>[9x]SELDSENDAADIAAGTIIAGAELTFGLLQNLLYFFANVNRKCAVGVDNESGFRWQEGSTYFFSGTADENLPYSVSDGYAVLYGPRKTNGPVATGVVGVLAYYIPSIGKTLAVMW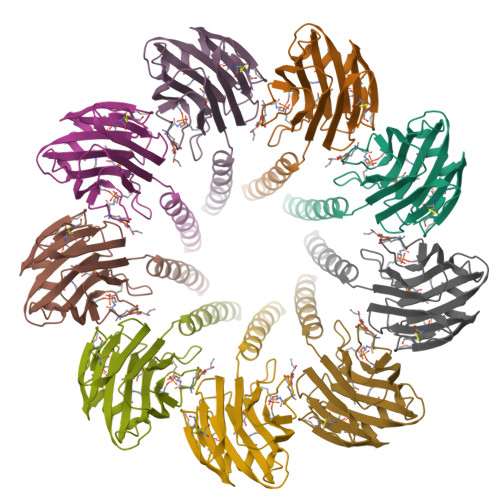SVPFDYNFYQNWWNAKLYSGNQRADYDHYVDLYYNANPFKANGWHERSLGSGLKFCGSMSSSGQATLEIHVLKESETCM>[2x]MMLSATQPLSEKLPAHGCRHVAIIMDGNGRWAKKQGKIRAFGHKAGAKSVRRAVSFAANNGIEALTLYAFSSENWNRPAQEVSALMELFVWALDSE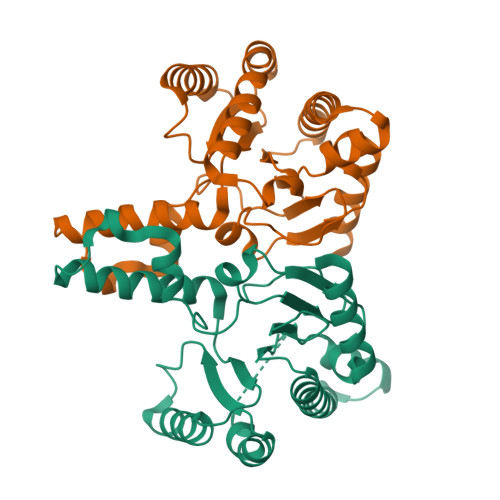VKSLHRHNVRLRIIGDTSRFNSRLQERIRKSEALTAGNTGLTLNIAANYGGRWDIVQGVRQLAEKVQQGNLQPDQIDEEMLNQHVCMHELAPVDLVIRTGGEHRISNFLLWQIAYAELYFTDVLWPDFDEQDFEGALNAFANRERRFGGTEPGDETA(5-methoxy-2-{[(4-methylphenyl)sulfonyl]carbamoyl}-1H-indol-1-yl)acetic 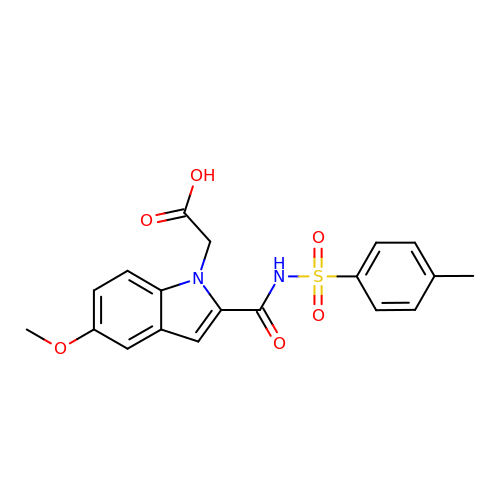acid | C19 H18 N2 O6 S | YJQRXPOQBVGZLN-UHFFFAOYSA-N> MSYSGERDNFAPHMALVPMVIEQTSRGERSFDIYSRLLKERVIFLTGQVEDHMANLIVAQM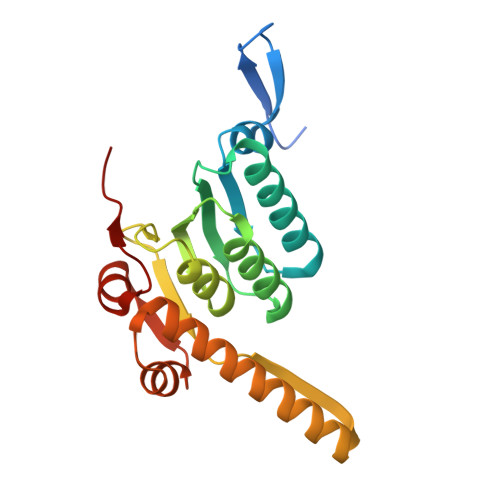LFLEAENPEKDIYLYINSPGGVITAGMSIYDTMQFIKPDVSTICMGQAASMGAFLLTAGAKGKRFCLPNSRVMIHQPLGGYQGQATDIEIHAREILKVKGRMNELMALHTGQSLEQIERDTERDRFLSAPEAVEYGLVDSILTHRN DSFs are a family of fatty acid AIs produced and detected by a wide range of gram-negative bacteria, including important pathogens. The DSF receptor RpfR is conserved in numerous gram-negative bacteria, including, among others, Escherichia coli, B. cenocepacia, Cronobacter turicensis, Serratia marcescens, Yersinia enterocolitica, and Enterobacter cloacae. RpfR was predicted to contain three domains, namely Per-Arnt-Sim (PAS), diguanylate cyclase (DGC), and phosphodiesterase (PDE) domains. BDSF binding to RpfR was previously shown to trigger its PDE activity, decreasing the intracellular concentration of c-di-GMP and favoring biofilm dispersal.

Without adding fatty acid to the crystallization experiment, we observed prominent electron density in the PAS domain core that was consistent with a 12-carbon fatty acid ligand. Intriguingly, even when an excess of BDSF was included during crystallization, the electron density was consistent with a fatty acid that did not contain a cis-2 double bond. These data suggested that RpfRCt(PAS) copurified with a tightly bound fatty acid likely originating from the E. coli overexpression host. Indeed, using liquid chromatography–mass spectrometry (LC-MS), we determined that the ligand is the saturated isomer of BDSF, C12:0, which E. coli is known to produce endogenously. Thus, we built and refined the 1.5 Å resolution X-ray crystal structure of RpfRCt(PAS)–C12:0. In the RpfRCt(PAS)–C12:0 structure, the C12:0 carboxylic acid group forms multiple hydrogen bonds with a set of conserved hydrophilic residues (S169, N172, Y183, and R187) at one end of the ligand-binding pocket. At the other end of the pocket, the C12:0 hydrophobic acyl tail is surrounded by conserved hydrophobic residues. While C12:0 is an inactive isomer of BDSF, the RpfRCt(PAS)–C12:0 structure provided the first insight into how fatty acids interact with RpfR and proved to be important for comparative analysis. Comparison of the RpfRCt(PAS)–BDSF and RpfRCt(PAS)–C12:0 structures reveals that the ligands adopt different conformations, resulting from the absence or presence of the cis-2 double bond in C12:0 or BDSF, respectively. BDSF was shown to tightly bind RpfRBc (Kd = 877 nM), while C12:0 (Kd = 800 μM) and trans-2 dodecenoic acid (Kd = 150 μM) were found to weakly interact with the receptor. We propose that the more electron rich N202 amide nitrogen interacts with the electron deficient Cβ of BDSF. This interaction cannot occur for the fully saturated C12:0 and would be significantly weaker for trans-2 dodecenonic acid because its Cβ would be suboptimally positioned further away from N202.

> QVVSEANSVIVILDRHGNIQRFNRLSEEYTGLKEQEVIGQNVFTLFMSPAEASASRRNVTGFFRNGSSYEVERWIKTRKGQRLFLFRNKFVHSGSGRNEIFLICSGTDIT>[4x]CDLNINDDPNYPMNDQVTADLIFPSISASIASAVGGEIYNYAGFFAQYYEQKPESNQYNTLCEYTFTESSQQMDYSYRILFAGALEDAKQVLEKTTNPADRFATTILRAYAFQIMVDNTSDSPYSEALQGNANATPKWDTGETVYKGILGEIDAAEAALDGSGMDVPDLIFNKNIAQWKGFANALRLRMYLRFIDANIDAASYTEKVKTLVQNNEFFTGDVKLDCFLDETDKRNPWYNTNAVGLTGNHCAAYPLVSYLSSTGDPRIAYGISKTDADGKYVGQLPGGKTHMQSILGTDNWKNKNVSAIDYSIGATKPVYFFTQAELQFLIAEVYARFHNDDANAKSAYEAGVTADFAVRGFAGQENTILEGACAWSAASTQADKLNLIYMQKWVSLFYMDHMEAWSEIRRTDCPKLSSYSAAQIQASESVYTPGELVAPWTNGLEAGGLMKRMTYPLSARQQNVNTPAGVPGSTPVWWDIK;>MQTQEVAIKPNLKVVLRSDAQQIDEVVVTAMGIKRSEKALGYAATSVGGEKIAESRTSDVMSSLAGKIAGVQISSTSSDPGASNSVIIRGVSSLSGTNQPLYVVDGVPLNNSTVYSTDGLNSGYDFGNGANAINPDDVANMTILKGAAATALYGSRAANGVVMITTKSGRKEKGVGIEYNGGVQWSTVLRLPEFQNEFGMGWNGNHTELENGSWGPRFDGSMQLWGNVYNNSQKLKPYVAMPDNIKDFFDAGFRYSNSLSFNGATDKSDYYVSFSQISDDGMIPTDADSYDKYTFSARGSHKAGALTFSSSLNYAYQKNNFATTGQGLSMLNSLYQTPRDISIIGLEDQNDPFNTPGYYYTPYGVMNPYYILNNYLNEYESERFYGKFQLDYEFLKYFKFTYRMGLDTTTGQSDKGKPNLYALYYEGTPNGEGQGSSSPFSGETGQYSEQITRRREINQDIMVNFNMPVNDFNIN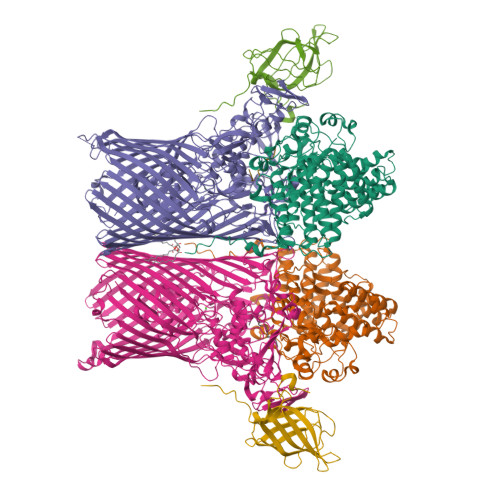ALVGFNGNERKVSYQYSEVNDLTIPTWFNLKNSGKTPIVEQHMELRRLMGVFGQFEGSWKNMLYLTVTARNDWSSTLPKENRSFFYPGITGSFIFSELLNDNLQDVITFGKIRASWGKTGNDADVYMVNPVYAQSSNRIPFGSLTFPLGGVNAYSAGNVLGSNTLSPEMTTESEVGLNMAFFKNRLSFDVSYYNRNTDKQIFSLAMDPASGYTAQNMNLGKIRNRGIELLISGTPIRTKDFSWELTWNFTKNWSKVISLPEELGGITTIYGLNGGTSMYAITGMPVGVFKAQVAERDPQGRIVVNSSTGLPVEASEFGICGDMNNKYQMGVSTNLKYKGISLGIDFDIRQGGVMYSRTKDINYFTGNAIQTAYNDRNPLIVPNSVNKIVNGENVTYVENTTPITSSNIYKYWGDGGSDMGSCFLVDKSYVKLRSVVLGWDLPKRWLAKTPFQAVKVSAYGNNLFVWTPSSNTFIDPEMTSFGNDLEGNYGEYTANPSSRRFGFNLMVKF[4x];>CDNDTEPGGTAVEKMAGDWWVTVNAFIDGKEVEDPFGAGHLQMSTYNTASNSETEMWLDDLGNFWEYKLKVNVNYAARTFSTTGFVDNVTYESKVKITDGKVLEKAATTPSGMPADSIVYMVQFDDDEDGLTYKVSGFRRTGFPADDF[4x];>[4x]GGGGGGGGGG> MG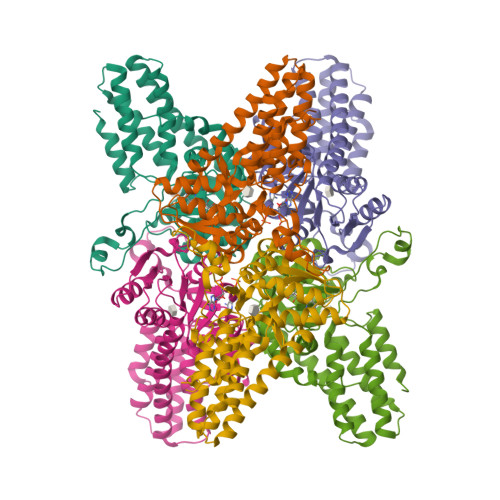AMIVKEVYETAEKIKSMEIRGAGRIARAAAQALMIQAEKSKAKEPEELWNELKVASKILYNTRPTAVSLPNALRYVMHRVKAAYLGGADLETLRFTAINSAKEFIYNSEKAIERIGEIGAKRIEDGDIIMTHCHSKAAISVMKKAFEQGKNIKVIVTETRPKWQGKITAKELASYGIPVIYIVDSAARHYMKMTDKVVMGANSITANGAVINKIGTSLIALTAKEHRVWVMIAAETYKFHPATMLGQLVEIEMRDPTEVIPEEELRTWPKNIEVWNPAFDVTPPEYIDVIITERGIIPPYAAIDILKEEFGWALKYKEPWED> MNTLPEHSCDVLIIGSGAAGLSLALRLADQHQVIVLSKGPVTEGSTFYAQGGIAAVFDETDSIDSHVEDTLIAGAGICDRHAVEFVASNARSCVQ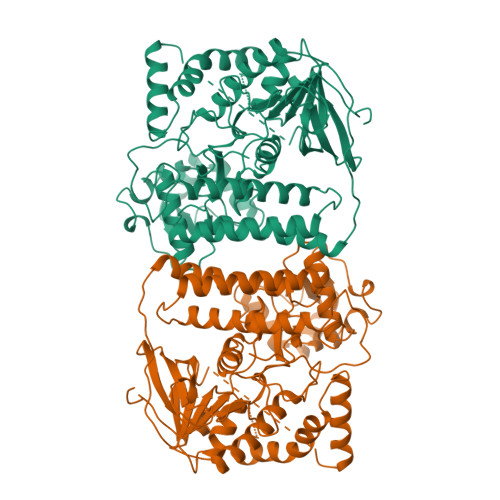WLIDQGVLFDTHIQPNGEESYHLTREGGHSHRRILHAADATGREVETTLVSKALNHPNIRVLERTNAVDLIVSDKIGLPGTRRVVGAWVWNRNKETVETCHAKAVVLATGGASKVYQYTTNPDISSGDGIAMAWRAGCRVANLEFNQFHPTALYHPQARNFLLTEALRGEGAYLKRPDGTRFMPDFDERGELAPRDIVARAIDHEMKRLGADCMFLDISHKPADFIRQHFPMIYEKLLGLGIDLTQEPVPIVPAAHYTCGGVMVDDHGRTDVEGLYAIGEVSYTGLHGANRMASNSLLECLVYGWSAAEDITRRMPYAHDISTLPPWDESRVENPDERVVIQHNWHELRLFMWDYVGIVRTTKRLERALRRITMLQQEIDEYYAHFRVSNNLLELRNLVQVAELIVRCAMMRKESRGLHFTLDYPELLTHSGPSILSPGNHYINR One of the most promising protein among various FAPs is the so-called FAST protein (“Fluorescence-Activating and absorption-Shifting Tag”),14 an engineered variant of the photoreceptor from Halorhodospira halophila – Photoactive Yellow Protein (PYP). This photoactive protein covalently binds a hydroxycinnamic acid. However, the replacement of several amino acids (including the key cysteine responsible for covalent binding) allowed using it as an FAP with a group of fluorogens. In this paper, using NMR spectroscopy and X-ray crystallography, we have studied the structure of fluorogen-activating protein FAST both in the apo form and in complex with the fluorogen.

Through the whole of our study, we crystallized the FAST protein several times, either in the presence of various ligands or without them. Surprisingly, we found that the protein adopts a form of the ligand-free domain-swapped dimer in crystals under a wide variety of conditions. In this dimer, the first three strands of the core β sheet (A30-L33, I39-N43, and T50-R52) are exchanged with the corresponding elements from the symmetrical molecule, forming together one large twelve-stranded β sheet (ESI Part 3†). Contrary to X-ray data and in good correlation with reported previously, both forms of protein are present in solution exclusively in the monomeric form (the determined hydrodynamic radius was 2.1 ± 0.1 nm, which corresponds to the 15 kDa).

> MEHVAFGSEDIENTLAKMDDGQLDGLAFGAIQLDGDGNILQYNAAEGDITGRDPKQVIGKNFFKDVAPGTDSPEFYGKFKEGVASGNLNTMFEWMIPTSRGPTKVKVHMKKALSGDSYWVFVKRVKLAAALEHHHHHH>MGMTNKASQPRTFTLSDEKRNHILTTALNLFDQFGFQHISIMRIITEAKIAKQSFYMAFPSKDSFIIECLDMEINRLKQSLSNLLGQCGKDDHTSILKSFYQWHVDLAYREGYNGTLLTKAVIEYWNLPDIKMKVEDFNKWKYEIFAEYLAEEINNARLRIIVSAMNGILLPA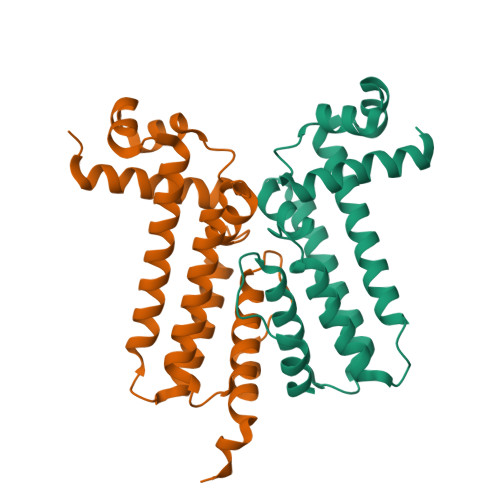STYLPTWEDIESLYGEQFHHHHHH[2x]4,4'-(2-aminopyridine-3,5-diyl)bis(2,6-difluorophenol) | C17 H10 F4 N2 O2 | 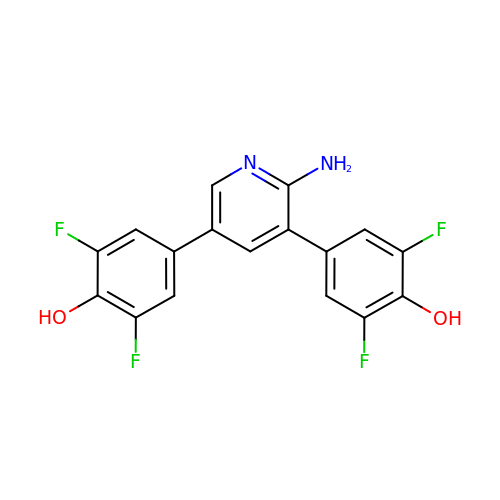FFWVPGLOKRROCI-UHFFFAOYSA-N5-[(4-{4-[(E)-2-cyanoethenyl]-2,6-dimethylphenoxy}pyrimidin-2-yl)amino]-2-[4-(methanesulfonyl)piperazin-1-yl]benzonitrile 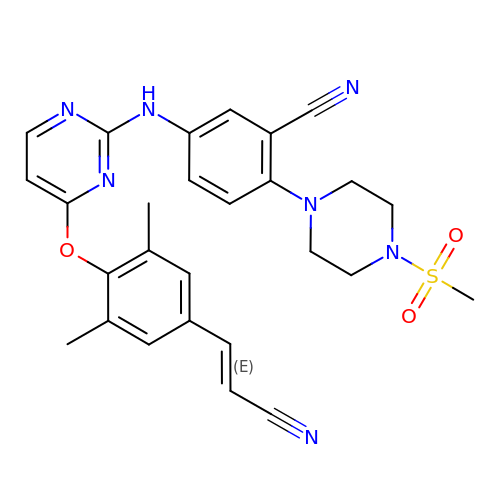| C27 H27 N7 O3 S | MMKBLGUSICHJOZ-SNAWJCMRSA-N> MGHHHHHHHHMATLTAKNLAKAYKGRRVVEDVSLT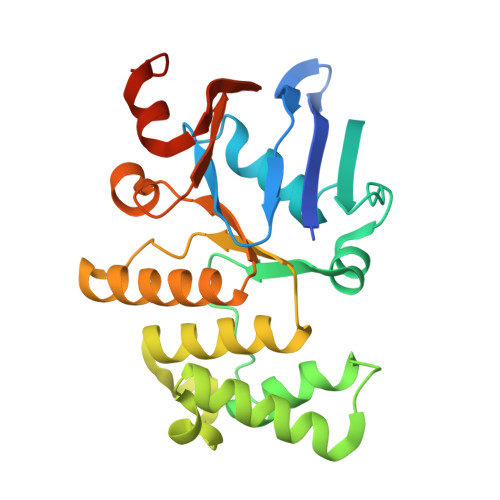VNSGEIVGLLGPNGAGKTTTFYMVVGIVPRDAGNIIIDDDDISLLPLHARARRGIGYLPQEASIFRRLSVYDNLMAVLQIRDDLSAEQREDRANELMEEFHIEHLRDSMGQSLSGGERRRVEIARALAANPKFILLDEPFAGVDPISVIDIKRIIEHLRDSGLGVLITDHNVRETLAVCERAYIVSQGHLIAHGTPTEILQDEHVKRVYLGEDFRL> FY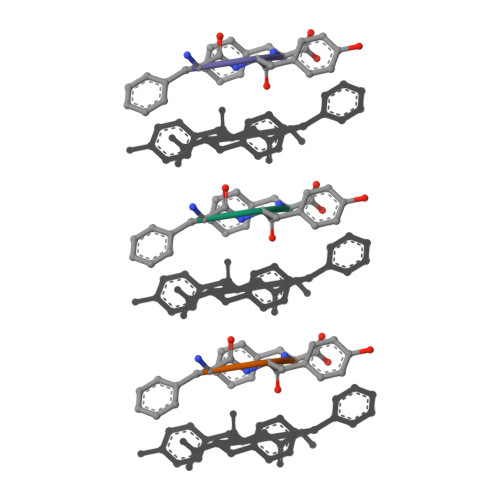F> MKLAIAALLATSAAAFTTSPASRATTSLQVSEIELGATEPLGVFDPLGWLETEPEAFERRRAVERKHGRVAMAAVVGTIVHNNHIVFDGYISPSNNLKFSDIPTGIDGIFSVPTAGLAQIIAFLGFVELAWLPASQYDGDYG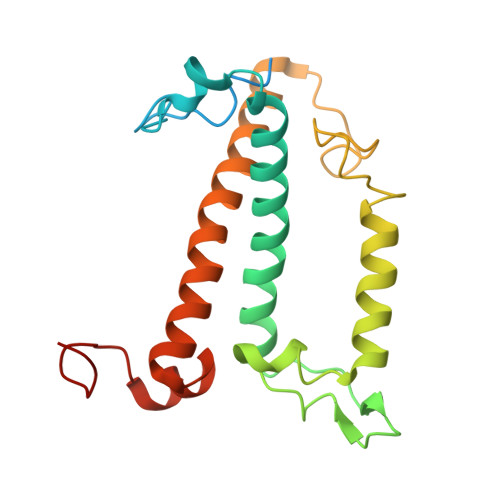VGYFGNDILDPEEKARKLNAELNNGRAAMMGIMGNMVAEKITGQTMYEQYAAGHFNPFNDGEGFF>[2x]MNGAIKVGAWGGNGGSAFDMGPAYRIISVKIFSGDVVDGVDVTFTYYGK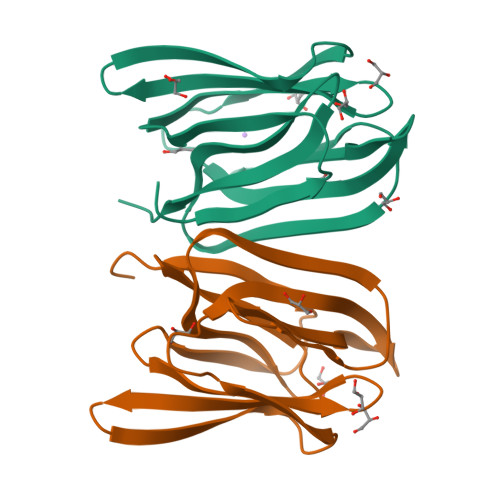TETRHYGGSGGTPHEIVLQEGEYLVGMAGEVANYTGAVVLGKLGFSTNKKAYGPFGNTGGTPFSLPIAAGKISGFFGRGGKFLDAIGVYLEPLA>[2x]GSHMAHAMENSWTISKEYHIDEEVGFALPNPQENLPDFYNDWMFIAKHLPDLIESGQLRERVEKLNMLSIDHLTDHKSQRLARLVLGCITMAYVWGKGHGDVRKVLPRNIAVPYCQLSKKLELPPILVYADCVLANWKKKDPNKPL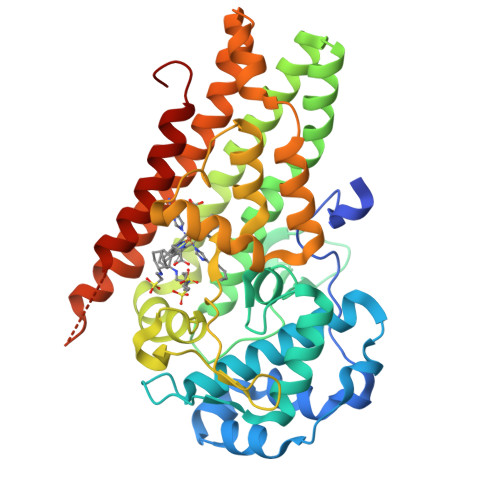TYENMDVLFSFRDGDCSKGFFLVSLLVEIAAASAIKVIPTVFKAMQMQERDTLLKALLEIASCLEKALQVFHQIHDHVNPKAFFSVLRIYLSGWKGNPQLSDGLVYEGFWEDPKEFGGGSAGQSSVFQCFDVLLGIQQTAGGGHAAQFLQDMRRYMPPAHRNFLCSLESNPSVREFVLSKGDAGLREAYDACVKALVSLRSYHLQIVTKYILIPASQQPKENKTSEDPSKLEAKGTGGTDLMNFLKTVRSTTEKSLLKEG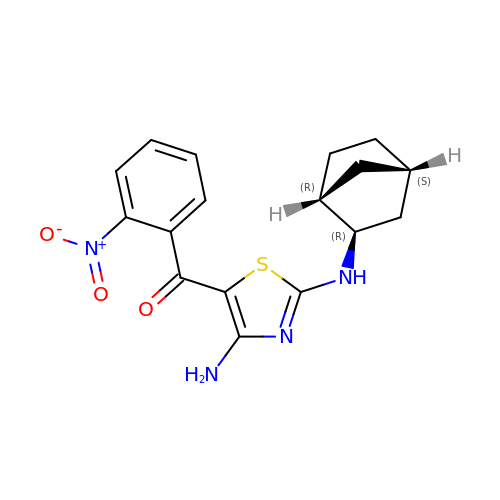(4-amino-2-{[(1R,2R,4S)-bicyclo[2.2.1]heptan-2-yl]amino}-1,3-thiazol-5-yl)(2-nitrophenyl)methanone | C17 H18 N4 O3 S | JRNXAQINDCOHGS-HOSYDEDBSA-N> M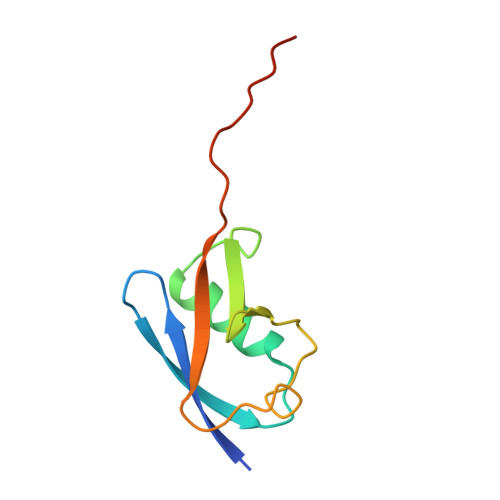ANDHINLKVAGQDGSVVQFKIKRHTPLSKLMKAYCERQGLSMRQIRFRFDGQPINETDTPAQLEMEDEDTIDVFQQQTGGVYLEHHHHHH> AAPGKPTIAWGNTKFAIVEVDQAATAYNNLVKVKNAADVSVSWNLWNGDTGTTAKILLNGKEAWSGPSTGSSGTANFKVNKGGRYQMQVALCNA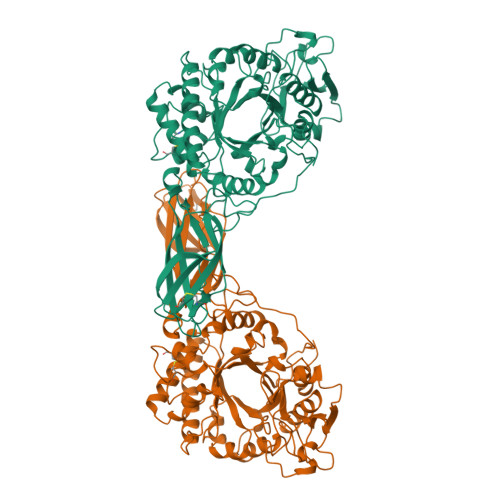DGCTASDATEIVVADTDGSHLAPLKEPLLEKNKPYKQNSGKVVGSYFVEWGVYGRNFTVDKIPAQNLTHLLYGFIPICGGNGINDSLKEIEGSFQALQRSCQGREDFKISIHDPFAALQKAQKGVTAWDDPYKGNFGQLMALKQAHPDLKILPSIGGWTLSDPFFFMGDKVKRDRFVGSVKEFLQTWKFFDGVDIDWEFPGGKGANPNLGSPQDGETYVLLMKELRAMLDQLSTETGRKYELTSAISAGKDKIDKVAYNVAQNSMDHIFLMSYDFYGAFDLKNLGHQTALNAPAWKPDTAYTTVNGVNALLAQGVKPGKIVVGTAMYGRGWTGVNGYQNNIPFTGTATGPVKGTWENGIVDYRQIAGQFMSGEWQYTYDATAEAPYVFKPSTGDLITFDDARSVQAKGKYVLDKQLGGLFSWEIDADNGDILNSMNASLGNSAGVQ2,4-DIAMINOBUTYRIC 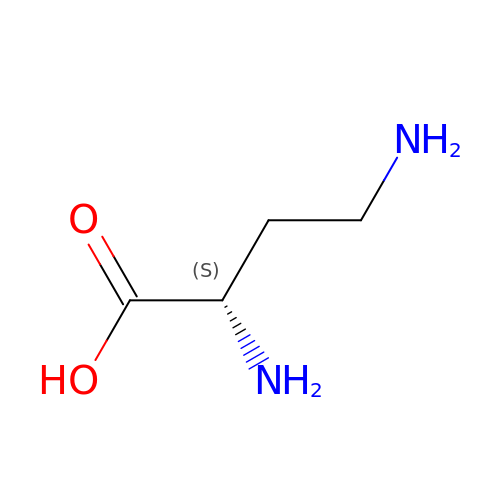ACID | C4 H10 N2 O2 | OGNSCSPNOLGXSM-VKHMYHEASA-N4'-[(3,6,9,12-tetraoxapentadec-14-yn-1-yl)oxy][1,1'-biphenyl]-4-yl sulfurofluoridate | C23 H27 F O8 S | 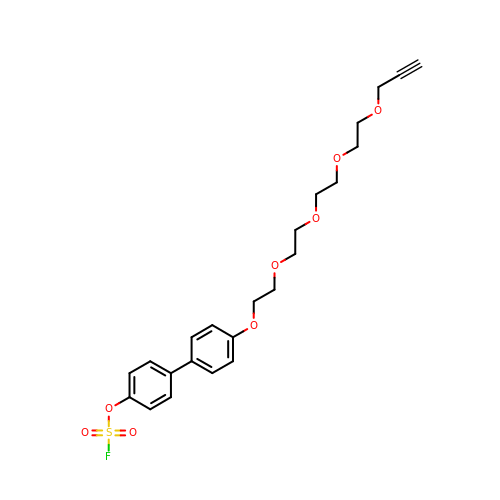LGGNGJGQVBUVOE-UHFFFAOYSA-N>[2x]MIVTVINQKGGVGKTTTSVNLSYYLSKEKKTGLLDLDPEGGATISYGMKRELKELPLGEKSVNIFNVEVFPAHIGLLKLELNGDVE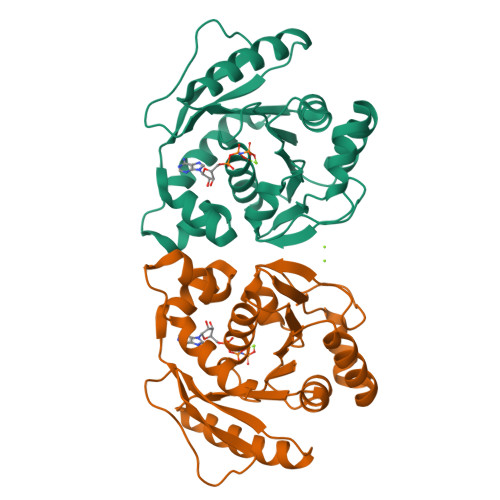EISNKIKEIGKQFDFLVIDTPPNLGTLAISAMLVADRIVSPVTPQPLALEAIKNLDSRLKSIGKNAYSFTNFSKKVVKLDNLSSVKFTEITIPPSRLFIEASRLGVPALRYEEVRIKKPKLANYYQQLAKVISE>[2x]MGSSHHHHHHSQDPMSLNLVSEQLLAANGLKHQDLFAILGQLAERRLDYGDLYFQSSYHESWVLEDRIIKDGSYNIDQGVGVRAISGEKTGFAYADQISLLALEQSAQAARTIVRDSGDGKVQTLGAVEHSPLYTSVDPLQSMSREEKLDILRRVDKVAREADKRVQEVTASLSGVYELILVAATDGTLAADVRPLVRLSVSVLVEEDGKRERGASGGGGRFGYEFFLADLDGEVRADAWAKEAVRMALVNLSAVAAPAGTMPVVLGAGWPGVLLHEAVGHGLEGDFNRRGTSVFSGQVGELVASELCTVVDDGTMVDRRGSVAIDDEGTPGQYNVLIENGILKGYMQDKLNARLMGMTPTGNGRRESYAHLPMPRMTNTYMLPGKSTPQEIIESVEYGIYAPNFGGGQVDITSDKFVFSTSEAYLIENGKVTKPVKGATLIGSGIETMQQISMVGNDLKLDNGVGVCGKEGQSLPVGVGQPTLKVDNLTVGGTA;>[2x]MALAMKVISQVEAQRKILEEAVSTALELASGKSDGAEVAVSKTTGISVSTRYGEVENVEFNSDGALGITVYHQNRKGSASSTDLSPQAIARTVQAALDIARYTSPDPCAGVADKELLAFDAPDLDLFHPAEVSPDEAIELAARAEQAALQADKRITNTEGGSFNSHYGVKVFGNSHGMLQGYCSTRHSLSSCVIAEENGDMERDYAYTIGRAMSDLQTPEWVGADCARRTLSRLSPRKLSTMKAPVIFANEVATGLFGHLVGAIAGGSVYRKSTFLLDSLGKQILPDWLTIEEHPHLLKGLASTPFDSEGVRTERRDIIKDGILTQWLLTSYSARKLGLKSTGHAGGIHNWRIAGQGLSFEQMLKEMGTGLVVTELMGQGVSAITGDYSRGAAGFWVENGEIQYPVSEITIAGNLKDMWRNIVTVGNDIETRSNIQCGSVLLPEMKIAGQ;>[2x]DRVY

Using a combination of biochemical and crystallographic methods we show that E. coli TldD and TldE interact to form a heterodimeric metalloprotease. TldD/E cleaves the N-terminal leader sequence from the modified MccB17 precursor peptide, to yield mature antibiotic, while it has no effect on the unmodified peptide. Both proteins are essential for the activity; however, only the TldD subunit forms a novel metal-containing active site within the hollow core of the heterodimer. Peptide substrates are bound in a sequence-independent manner through β sheet interactions with TldD and are likely cleaved via a thermolysin-type mechanism.

To explore the substrate binding site of the TldD/E heterodimer, wild-type or mutant (Glu263Ala) TldD/E was co-crystallized with a variety of peptides and peptide mimics, leading to four distinct ligand-bound complexes. Wild-type TldD/E crystals were grown in the presence of the peptide angiotensin II, and customized angiotensin II variant where the central (Tyr-Ile) peptide bond is replaced with a non-cleavable methylene bond, to yield two co-crystal structures with clear density for peptides where the carboxyl group of the C-terminal residue acts as a ligand to the catalytic zinc ion. In the case of angiotensin II, the density was consistent with Asp-Arg-Val-Tyr (hence WT-DRVY), indicative of cleavage at the central peptide bond of angiotensin. Using the standard nomenclature for protease active sites, these two ligands spanned subsites S4-S1 and S3-S1, respectively, occupying roughly half of the active site cleft. WT-DRVY peptide ligand was refined with occupancy of 0.7.> EG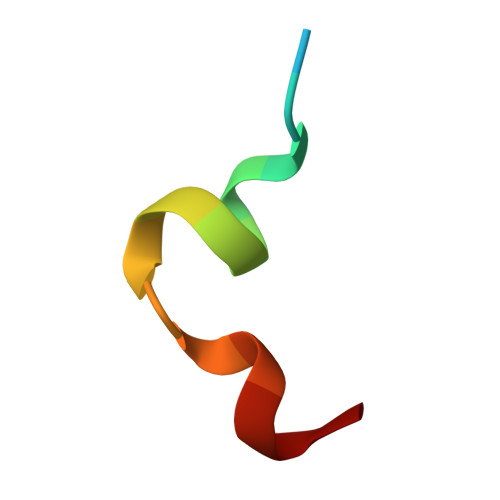DIPAIYRYGLEGLL>[2x]GEETRTEVEKKNYMNNAEEAKDVLLGVYRTNTLDAMYGYYLSILFNLGTDISQVEGSGNENFRIIPTNSFPTTQSEVQQTWAALYTGIYRANDFLERISNKIGSY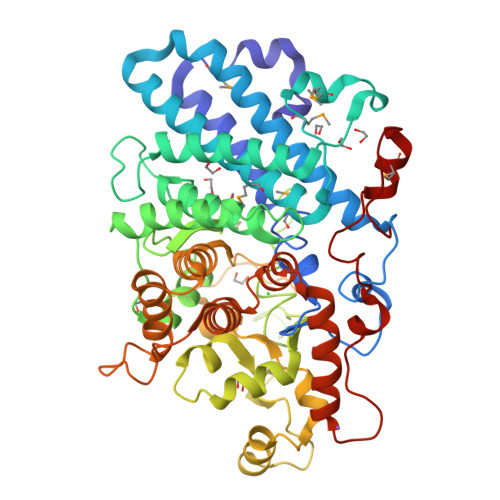TTTDKKLATLYIAEARALRGMFYFELVRRFGNVVLMTSTQMSNQNPATYVQSAPEKVYEYIEDDLLYACDILPYATDDQYRESNDYRFSKGAALGLLTKVYATWAGYPVKDESKWEAAAKTARILVESGKHGLLKDYEQLWKNTCNGTWDPTESLIEISFYSPTVSGNSDPVGRIGKWNGVKTTAIAGVRGSCAANVKVVHTFVLDWREDVSDIRRDLSIANYQYTDTKKSLWVAGASDTDESAAEKDADPTKAQKNKQNYTPAKWDIQKYVTTNSFINNDKSNVNWYFLRYADVLLLYAEALNEWKHGPDAEAYNAINAVRRRGYGNPSNTSACDLPQGLDETSFREAVRKERSYELSFEGHRRQDLIRWGIYYKTVQATAKELGYWWEGTGSPNYSVATYTEEGKHELFPIPQRDMDLCIQFNQNPKW> MTKLQPNTVIRAALDLLNEVGVDGLTTRKLAERLGVQQPALYWHFRNKRALLDALAEAMLA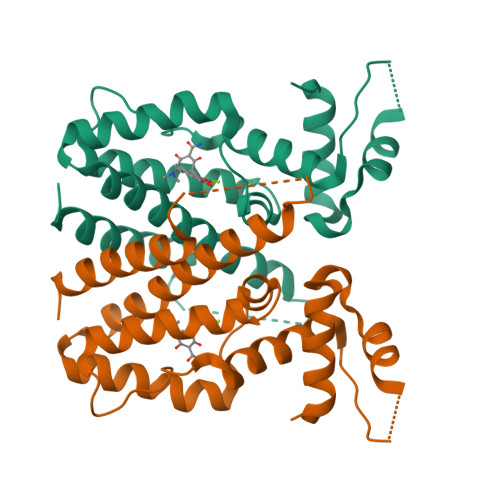ENHSTSVPRADDDWRSFLTGNARSFRQALLAYRDGARIHAGTRPGAPQMETADAQLRFLCEAGFSAGDAVNALMTISYFTVGAVLEEQAGDSESGERGGTVEQAPLSPLLRAAIDAFDEAGPDAAFEQGLAVIVDGLAKRRLVVRNVEGPRKGDD ALPHA-FLUORO-CARBOXYMETHYLDETHIA COENZYME A COMPLEX 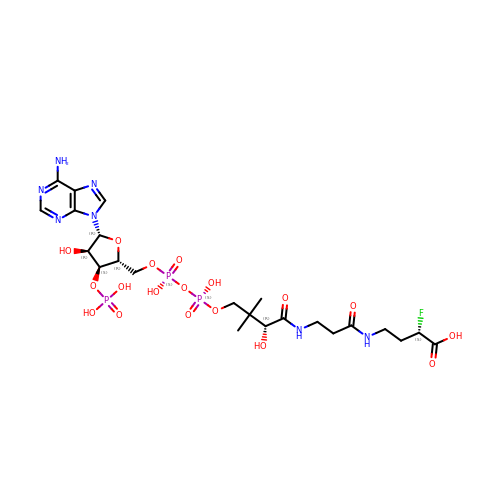| C23 H37 F N7 O18 P3 | JYRBBNPCUSRRNJ-KFJQBOOGSA-N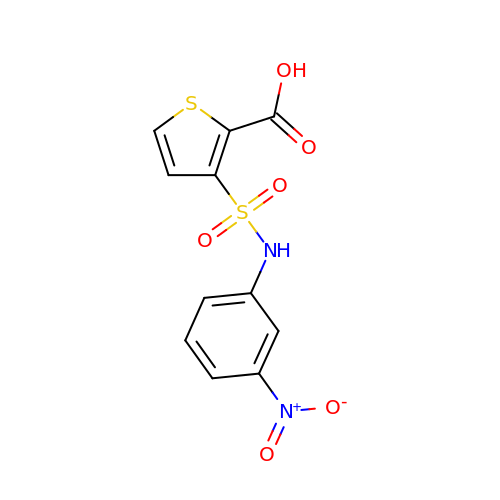3-{[(3-NITROANILINE]SULFONYL}THIOPHENE-2-CARBOXYLIC ACID | C11 H8 N2 O6 S2 | CITCNTPVKZFUAJ-UHFFFAOYSA-N>[12x]XGKLEALAQK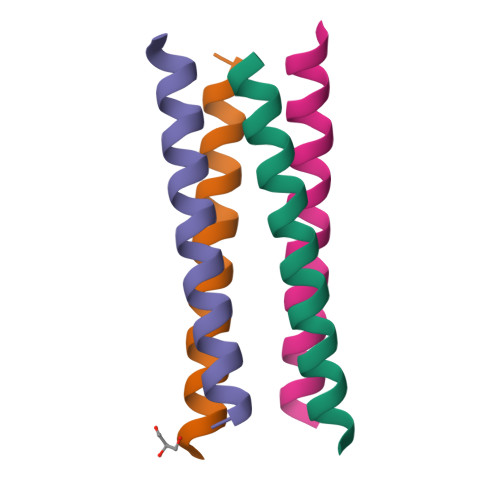LEALAKKLEALAWKLEALAQGX>SNAMRWNICVVGAGKIGQMIAALLKTSSNYSVTVADHDLAALAVLNRMGVATKQVDAKDEAGLAKALGGFDAVISAAPFFLTPIIAKAAKAAGAHYFDLTEDV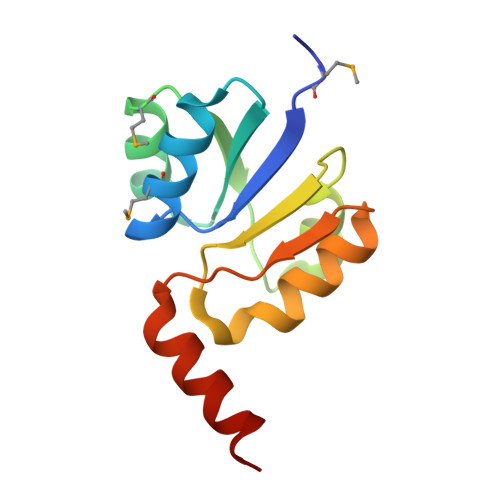AATNAVRALVEDSQT[2x]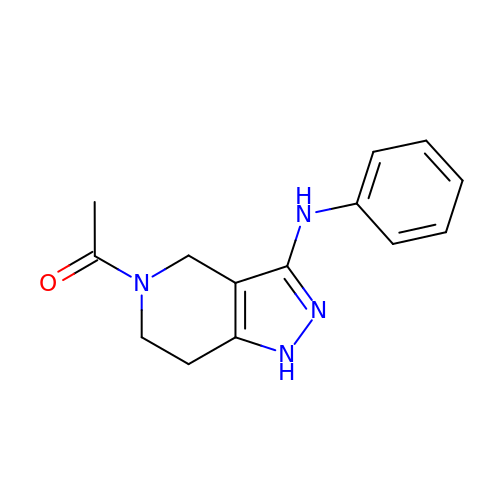1-(3-phenylazanyl-1,4,6,7-tetrahydropyrazolo[4,3-c]pyridin-5-yl)ethanone | C14 H16 N4 O | ZXIJCVCJLDGJRX-UHFFFAOYSA-N> SEEDVVKMSPLPTVENQFTPTTAWSTSVGSGIGNFYSNLHPALADNVVYAADRAGLVKALNADDGKEIWSVSLAEKDGWFSKEPALLSGGVTVSGGHVYIGSEKAQVYALNTSDGTVAWQTKVAGEALSRPVVSDGLVLIHTSNGQLQALNEADGAVKWTVNLDMPSLSLRGESAPTTAFGAAVVGGDNGRVSAVLMEQGQMIWQQRISQATGSTEIDRLSDVDTTPVVVNGVVFALAYNGNLTALDLRSGQIMWKRELGSVNDFIVDGNRIYLVDQNDRVMALTIDGGVTLWTQSDLLHRLLTSPVLYNGNLVVGDSEGYLHWINVEDGRFVAQQKVDSSG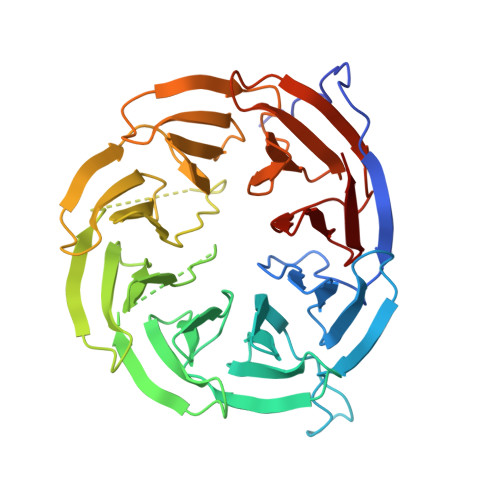FQTEPVAADGKLLIQAKDGTVYSITR>MVVPESFQLDQEILLDAGAQLHRLKMYPYFDVAH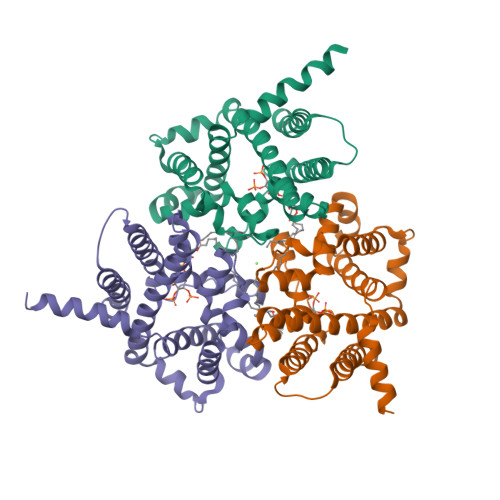YLLMIIEVRDDLGSAASIFSRKHPLSCWLSSMLMCFADAFLANFLLGEPVIAPFKRHDDIILATIIWYLVFYAPFDGIYKIAKITPVKCVLAVMKEVKRAYKVSHGVSHAAKLYPNSYIVQVLVGTAKGAGSGIVRTLEQLVRGVWLPTHNELLRPSFATKACVVAASVLALEKSGTYLTAPHDLVYLVIVGFFVYFKLSAVILHVTDPFAPIENLFHHHHHH[3x]>[2x]GQVSKTYYVSKPGTLISMMTEEEANSITHLTLTGKLNAEDFRHLRDEFPSLKVLDISNAEIKMYSGKAGTYPNGKFYIYMANFVPAYAFSNVVNGVTKGKQTLEKVILSEKIKNIEDAAFKGCDNLKICQIRKKTAPNLLPEALADSVTAIFIPLGS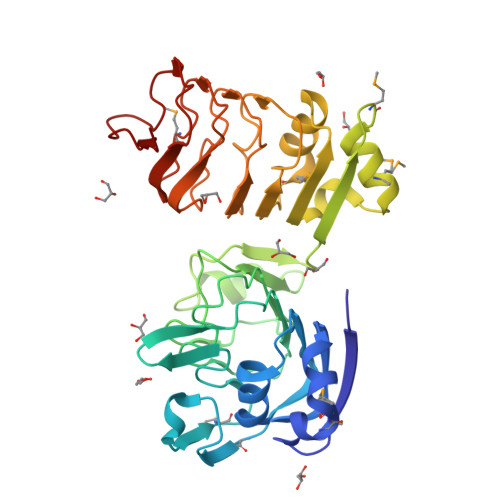SDAYRFKNRWEHFAFIEGEPLETTIQVGAMGKLEDEIMKAGLQPRDINFLTIEGKLDNADFKLIRDYMPNLVSLDISKTNATTIPDFTFAQKKYLLKIKLPHNLKTIGQRVFSNCGRLAGTLELPASVTAIEFGAFMGCDNLRYVLATGDKITTLGDELFGNGVPSKLIYKK> GDRVADVIESSIGDSVSRALTHALPAPTGQDTQVSSHRLDTGKVPALQAAEIGASSNASDESMIETRCVLNSHSTAETTLDSFFSRAGLVGEIDLPLKGTTNPNGYANWDIDITGYAQMRRKVELFTYMRFDAEFTFVACTPTGEVVPQLLQYMFVPPGAPKPDSRESL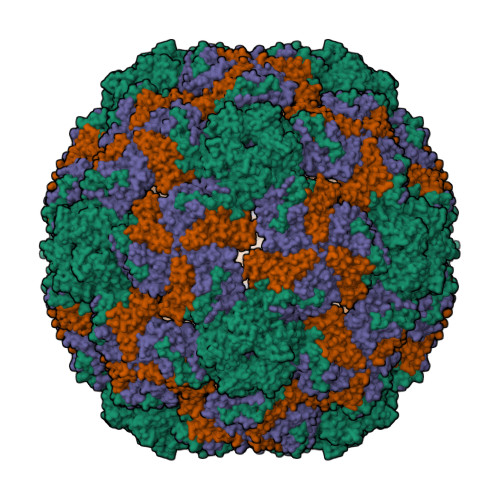AWQTATNPSVFVKLSDPPAQVSVPFMSPASAYQWFYDGYPTFGEHKQEKDLEYGACPNNMMGTFSVRTVGTSKSKYPLVVRIYMRMKHVRAWIPRPMRNQNYLFKANPNYAGNSIKPTGTSRTAITTL;> SPSAEACGYSDRVAQLTIGNSTITTQEAANIIVGYGEWPSYCSDSDATAVDKPTRPDVSVNRFYTLDTKLWEKSSKGWYWKFPDVLTETGVFGQNAQFHYLYRSGFCIHVQCNASKFHQGALLVAVLPEYVIGTVAGGTGTEDSHPPYKQTQPGADGFELQHPYVLDAGIPISQLTVCPHQWINLRTNNCATIIVPYINALPFDSALNHCNFGLLVVPISPLDYDQGATPVIPITITLAPMCSEFAGLRQAVTQ;> GFPTELKPGTNQFLTTDDGVSAPILPNFHPTPCIHIPGEVRNLLELCQVETILEVNNVPTNATSLMERLRFPVSAQAGKGELCAVFRADPGRNGPWQSTLLGQLCGYYTQWSGSLEVTFMFTGSFMATGKMLIAYTPPGGPLPKDRATAMLGTHVIWDFGLQSSVTLVIPWISNTHYRAHARDGVFDYYTTGLVSIWYQTNYVVPIGAPNTAYIIALAAAQKNFTMKLCKDASDILQTGTIQ>MAHHHHHHSAALEVLFQGPGMAETKLQLFVKASEDGESVGHCPSCQRLFMVLLLKGVPFTLTTVDTRRSPDVLKDFAPGSQLPILLYDSDAKTDTLQIEDFLEETLGPPDFPSLAPRYRESNTAGNDVFHKFSAFIKNPVPAQDEALYQQLLRALARLDSYLRAPLEHELAGEPQLRESRRRFLDGDRLTLADCSLLPKLHIVDTVCAHFRQAPIPAELRGVRRYLDSAMQEK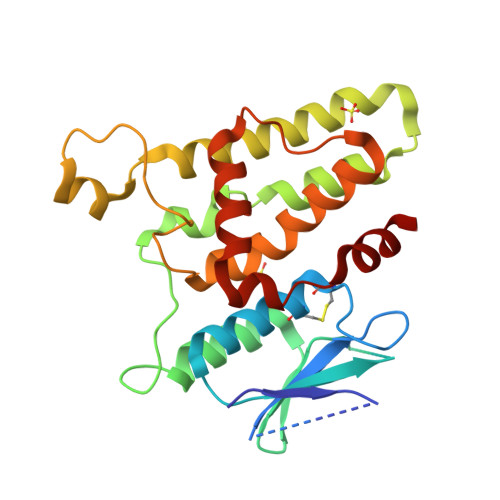EFKYTCPHSAEILAAYR[2x]>MGHHHHHHMNSVKNEENTSKEHAPDKIVLDHAFGQTILDK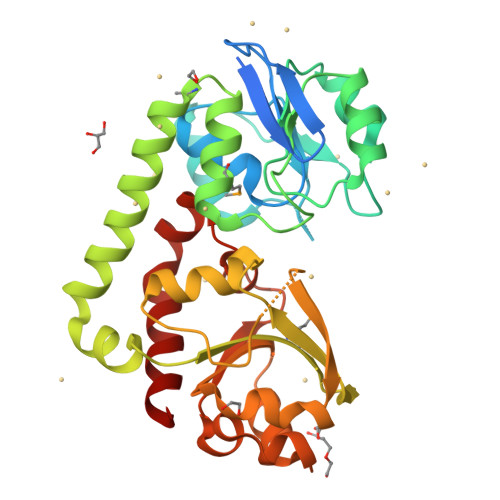KPERVATIAWGNHDVALALGIVPVGFSKANYGVSADKGVLPWTEEKIKELNGKANLFDDLDGLNFEAISNSKPDVILAGYSGITKEDYDTLSKIAPVAAYKSKPWQTLWRDMIKIDSKALGMEKEGDELIKNTEARISKELEKHPEIKGKIKGKKVLFTMINAADTSKFWIYTSKDPRANYLTDLGLVFPESLKEFESEDSFAKEISAEEANKINDADVIITYGDDKTLEALQKDPLLGKINAIKNGAVAVIPDNTPLAASCTPTPLSINYTIEEYLNLLGNACKNAK[2x]> GPLGSMGTPQKDVIIKSDAPDTLLLEKHADYIASYGSKKDDYEYCMSEYLRMSGIYWGLTVMDLMGQLHRMNREEILAFIKSCQHECGGISASIGHDPHLLYTLSAVQILTLYDSINVIDVNKVVEYVKGLQKEDGSFAGDIWGEIDTRFSFCAVATLALLGKLDAINVEKAIEFVLSCMNFDGGFGCRPGSESHAGQIYCCTGFLAITSQLHQVNSDLLGWWLCERQLPSGGLNGRPEKLPDVCYSWWVLASLKIIGRLHWIDREKLRNFILACQDEETGG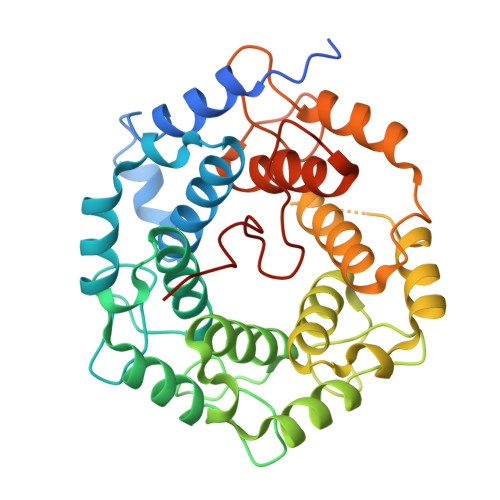FADRPGDMVDPFHTLFGIAGLSLLGEEQIKPVNPVFCMPEEVLQRVNVQPELVS> MSHTILLVQPTKRPEGRTYADYESVNE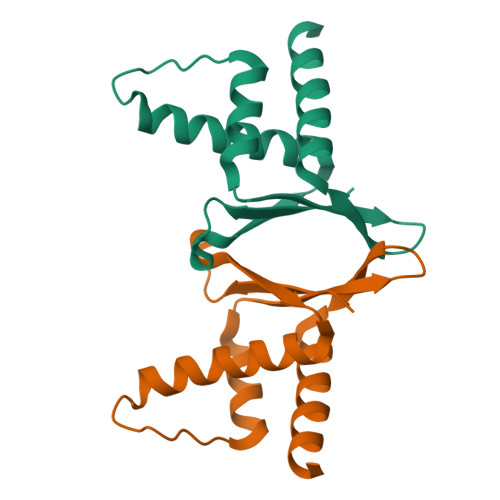CMEGVCKMYEEHLKRMNPNSPSITYDISQLFDFIDDLADLSCLVYRADTQTYQPYNKDWIKEKIYVLLRRQAQQAGK> MLEKFCNSTFWNSSFLDSPEADLPLCFEQTVLVWIPLGYLWLLAPWQLLHVYKSRTKRSSTTKLYLAKQVFVGFLLILAAIELALVLTEDSGQATVPAVRYTNPSLYLGTWLLVLLIQYSRQWCVQKNSWFLSLFWILSILCGTFQFQTLIRTLLQGDNSNLAYSCLFFISYGFQILILIFSAFSENNESSNNPSSIASFLSSITYSWYDSIILKGYKRPLTLEDVWEVDEEMKTKTLVSKFETHMKRELQKARRALQRRQEKSSQQNSGARLPGLNKNQSQSQDALVLEDVEKKKKKSGTKKDVPKSWLMKALFKTFYMVLLKSFLLKLVNDIFTFVSPQLLKLLISFASDRDTYLWIGYLCAILLFTAALIQSFCLQCYFQLCFKLGVKVRTAIMASVYKKALTLSNLARKEYTVGETVNLMSVDAQKLMDVTNFMHMLWSSVLQIVLSIFFLWRELGPSVLAGVGVMVLVIPINAILSTKSKTIQVKNMKNKDKRLKIMNEILSGIKILKYFAWEPSFRDQVQNLRKKELKNLLAFSQLQCVVIFVFQLTPVLVSVVTFSVYVLVDSNNILDAQKAFTSITLFNILRFPLSMLPMMISSMLQASVSTERLEKYLGGDDLDTSAIRHDCNFDKAMQFSEASFTWEHDSEATVRDVNLDIMAGQLVAVIGPVGSGKSSLISAMLGEMENVHGHITIKGTTAYVPQQSWIQNGTIKDNILFGTEFNEKRYQQVLEACALLPDLEMLPGGDLAEIGEKGINLSGGQKQRISLARATYQNLDIYLLDDPLSAVDAHVGKHIFNKVLGPNGLLKGKTRLLVTHSMHFLPQVDEIVVLGNGTIVEKGSYSALLAKKGEFAKNLKTFLRHTGPEEEATVHDGSEEEDDDYGLISSVEEIPEDAASITMRRENSFRRTLSRSSRSNGRHLKSLRNSLKTRNVNSLKEDEELVKGQKLIKKEFIETGKVKFSIYLEYLQAIGLFSIFFIILAFVMNSVAFIGSNLWLSAWTSDSKIFNSTDYPASQRDMRVGVYGALGLAQGIFVFIAHFWSAFGFVHASNILHKQLLNNILRAPMRFFDTTPTGRIVNRFAGDISTVDDTLPQSLRSWITCFLGIISTLVMICMATPVFTIIVIPLGIIYVSVQMFYVSTSRQLRRLDSVTRSPIYSHFSETVSGLPVIRAFEHQQRFLKHNEVRIDTNQKCVFSWITSNRWLAIRLELVGNLTVFFSALMMVIYRDTLSGDTVGFVLSNALNITQTLNWLVRMTSEIETNIVAVERITEYTKVENEAPWVTDKRPPPDWPSKGKIQFNNYQVRYRPELDLVLRGITCDIGSMEKIGVVGRTGAGKSSLTNCLFRILEAAGGQIIIDGVDIASIGLHDLREKLTIIPQDPILFSGSLRMNLDPFNNYSDEEIWKALELAHLKSFVASLQLGLSHEVTEAGGNLSIGQRQLLCLGRALLRKSKILVLDEATAAVDLETDNLIQTTIQNEFAHCTVITIAHRLHTIMDSDKVMVLDNGKIIECGSPEELLQIPGPFYFMAKEAGIENVNSTKF

Multidrug resistance-associated protein 2 (MRP2) is an ATP-powered exporter important for maintaining liver homeostasis and a potential contributor to chemotherapeutic resistance. MRP2 is a single polypeptide comprising of an N-terminal transmembrane domain (TMD0) and the canonical transporter core of two transmembrane domains (TMD1 and TMD2) and two nucleotide-binding domains (NBD1 and NBD2). Using cryogenic electron microscopy (cryo-EM), we determine the structures of human MRP2 in three conformational states: an autoinhibited state, a substrate-bound pre-translocation state, and an ATP-bound post-translocation state.

To understand how substrate is recognized by MRP2 and the effect of substrate binding on the autoinhibitory R domain, we determined the cryo-EM structure of WT MRP2 in the presence of leukotriene C4 (LTC4), a pro-inflammatory signaling molecule that is transported by multiple MRP transporters. Cryo-EM reconstruction obtained in the presence of 40 μM LTC4 revealed the same structure as the auto-inhibited state; only in the presence of 285 μM LTC4 were we able to observe clear density for LTC4 in the substrate-binding site. The cryo-EM map, refined to an overall resolution of 2.75 Å, shows no density for the R domain, indicating that the R domain is flexible in this conformation. These results suggest that only at sufficiently high concentrations can the substrate displace the R domain to be transported. LTC4 binds at the interface of the two TM bundles, triggering a global conformational change that brings the two halves of the transporter core closer together. The inward-swing of the NBDs originates at the substrate-binding site, where TM helix 6, 8, 16, and 17 move towards each other and the side chains of F591 and W1254 reposition to contact LTC4. In MRP2, LTC4 is largely stabilized by hydrogen bonds between the GSH moiety and residues K329, Q447, R1205, and R1257. Despite the high resolution of the cryo-EM map and clear density for the GSH moiety, density for the lipid tail is mostly absent except for a short portion stabilized by van der Waals interactions with W1254. In MRP2, the corresponding residue to Y440 is, in fact, a phenylalanine (F437), mirroring the Y440F variant of MRP1. Substrate displaces the R domain, permitting conformational changes necessary for transport.>[2x]STQYETQGYTINNAGRRLVVDPITRIEGHMRCEVNINDQNVITNAVSCGTMFRGLEIILQGRDPRDAWAFVERICGVCTGVHALASVYAIEDAIGIKVPDNANIIRNIMLATLWCHDHLVHFYQLAGMDWIDVLDALKADPRKTSELAQSLSSWPKSSPGYFFDVQNRLKKFVEGGQLGIFRNGYWGHPQYKLPPEANLMGFAHYL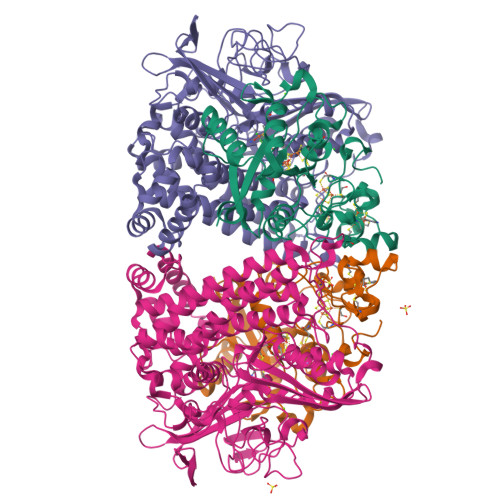EALDFQREIVKIHAVFGGKNPHPNWIVGGMPCAINIDESGAVGAVNMERLNLVQSIITRTADFINNVMIPDALAIGQFNKPWSEIGTGLSDKCVLSYGAFPDIANDFGEKSLLMPGGAVINGDFNNVLPVDLVDPQQVQEFVDHAWYRYPNDQVGRHPFDGITDPWYNPGDVKGSDTNIQQLNEQERYSWIKAPRWRGNAMEVGPLARTLIAYHKGDAATVESVDRMMSALNLPLSGIQSTLGRILCRAHEAQWAAGKLQYFFDKLMTNLKNGNLATASTEKWEPATWPTECRGVGFTEAPKGALGHWAAIRDGKIDLYQCVVPTTWNASPRDPKGQIGAYEAALMNTKMAIPEQPLEILRTLHSFDPCLACSTH;>KPRIPVVWIHGLECTCCTESFIRSAHPLAKDVILSLISLDYDDTLMAAAGTQAEEVFEDIITQYNGKYILAVEGNPPLGEQGMFCISSGRPFIEKLKRAAAGASAIIAWGTCASWGCVQAARPNPTQATPIDKVITDKPIIKVPGCPPIPDVMSAIITYMVTFDRLPDVDRMGRPLMFYGQRIHDKCYRRAHFDAGEFVQSWDDDAARKGYCLYKMGCKGPTTYNACSSTRWNDGVSFPIQSGHGCLGCAENGFWDRGSFYSRV[2x]>[2x]ALTYRGADISSLLLLEDEGYSYKNLNGQTQALETILADAGINSIRQRVWVNPSDGSYDLDYNLELAKRVKAAGMSLYLDLHLSDTWADPSDQTTPSGWSTTDLGTLKWQLYNYT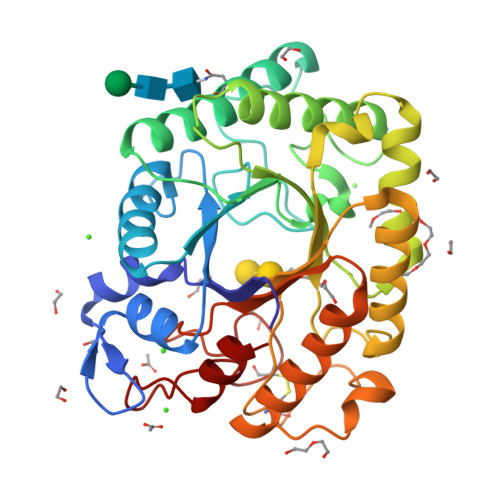LEVCNTFAENDIDIEIISIGNEIRAGLLWPLGETSSYSNIGALLHSGAWGVKDSNLATTPKIMIHLDDGWSWDQQNYFYETVLATGELLSTDFDYFGVSYYPFYSASATLASLKTSLANLQSTYDKPVVVVETNWPVSCPNPAYAFPSDLSSIPFSVAGQQEFLEKLAAVVEATTDGLGVYYWEPAWIGNAGLGSSCADNLMVDYTTDEVYESIETLGEL>[2x]MYGLVNKAIQDMISKHHGEDTWEAIKQKAGLEDIDFFVGMEAYSDDVTYHLVGAASEVLGKPAEEWLIAFGEYWVTYTSEEGYGELLASAGDSLPEFMENLDNLHARVGLSFPQLRP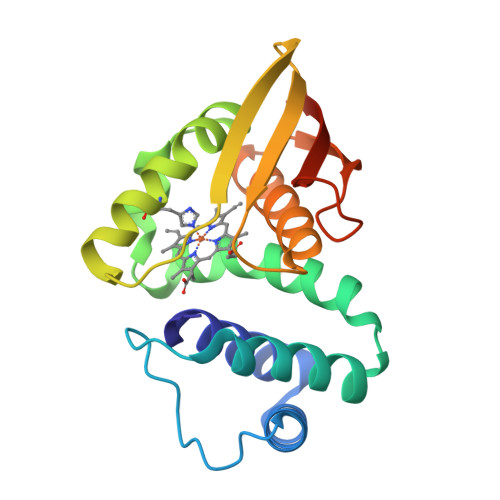PAFECQHTSSKSMELHYQSTRCGLAPMVLGLLHGLGKRFQTKVEVTQTAFRETGEDHDIFSIKYEDSNLYDD>KDYDAYLSYTKVDPDQWNQETGEEERFALEILPDMLEKHYGYKLFIPDRDLIPTGTYIEDVARCVDQSKRLIIVMTPNYVVRRGWSIFELETRLRNMLVTGEIKVILIE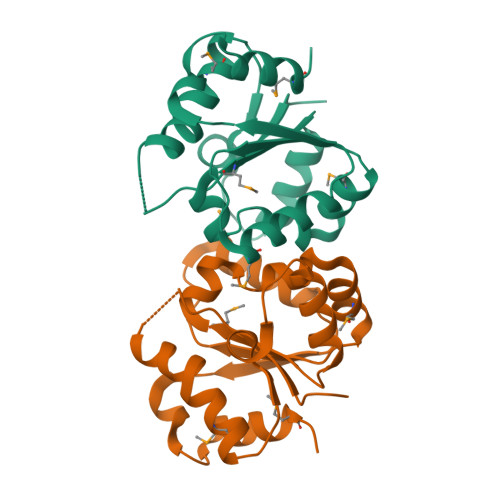CSELRGIMNYQEVEALKHTIKLLTVIKWHGPKCNKLNSKFWKRLQYEMPF[2x]(2S)-5-hydroxy-2-(4-hydroxyphenyl)-7-methoxy-2,3-dihydro-4H-chromen-4-one | C16 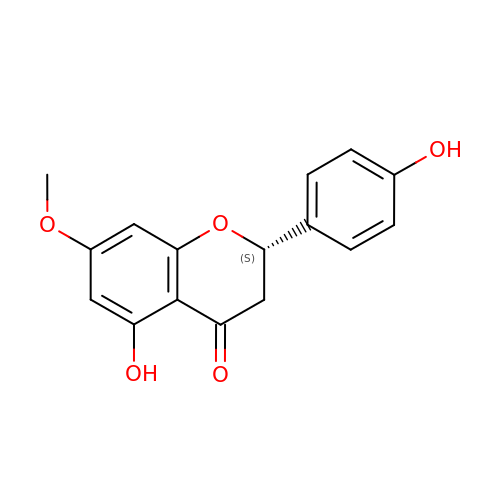H14 O5 | DJOJDHGQRNZXQQ-AWEZNQCLSA-N> SLMVLAMESRVAPEIPGLIQPGNVTQDLKMMVCKLLNSPKPTKTFPGSQPVSFQHSDVEEKLLAHDYYVCEKTDGLRVLMFIVINPVTGEQGCFMIDRENNYYLVNGFRFPRLPQKKKEELLETLQDGTLLDGELVIQTNPMTKLQELRYLMFDCLAINGRCLTQSPTSSRLAHLGKEFFKPYFDLRAAYPNRCTTFPFKISMKHMDFSYQLVKVAKSLDKLPHLSDGLIFTPVKAPYTAGGKDSLLLKWKPEQENTVDFKLILDIPMVEDPSLPKDDRNRWYYNYDVKPVFSLYVWQGGADVNSRLKHFDQPFDRKEFEILERTYRKFAELSVSDEEWQNLKNLEQPLNGRIVECAKNQETGAWEMLRFRDDKLNGNHTSVVQKVLESINDSVSLEDLEEIVGDIKRCWDERRANMAGGSGRPLPSQSQN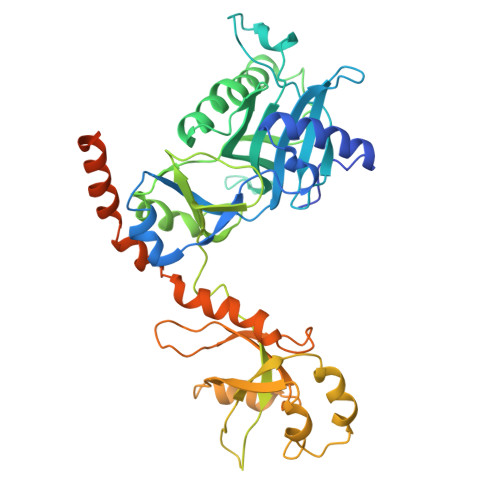ATLSTSKPVHSQPPSNDKEPKYVDEDDWSD>[6x]GSPASGTSLSAAIHRTQLWFHGRISREESQR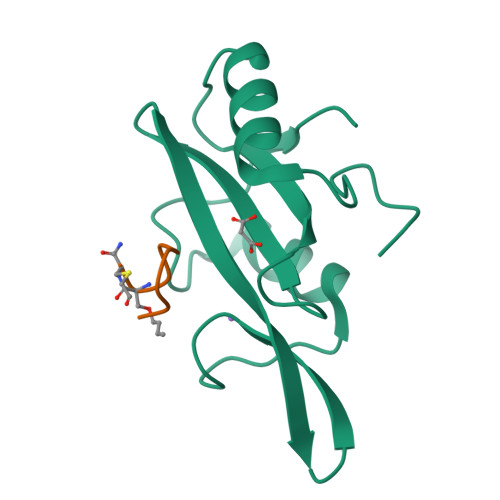LIGQQGLVDGLFLVRESQRNPQGFVLSLCHLQKVKHYLILPSEEEGRLYFSMDDGQTRFTDLLQLVEFHQLNRGILPCLLRHCCTRVAL;>[6x]SFEGYDNXC> MDLTVEPNLHSLITSTTHKWIFVGGKGGVGKTTSSCSIAIQMALSQPNKQFLLISTDPAHNLSDAFGEKFGKDARKVTGMNNLSCMEIDPSAALKDMNDMAVSRANNNGSDGQGDDLGSLLQGGALADLTGSIPGIDEALSFMEVMKHIKRQEQDEGETFDTVIFDTAPTGHTLRFLQLPNTLSKLLEKFGEITNKLGPMLNSFMGAGNVDISGKLNELKANVETIRQQFTDPDLTTFVCVCISEFLSLYETERLIQELISYDMDVNSIIVNQLLFAENDQEHNCKRCQARWKMQKKYLDQIDELYEDFHVVKMPL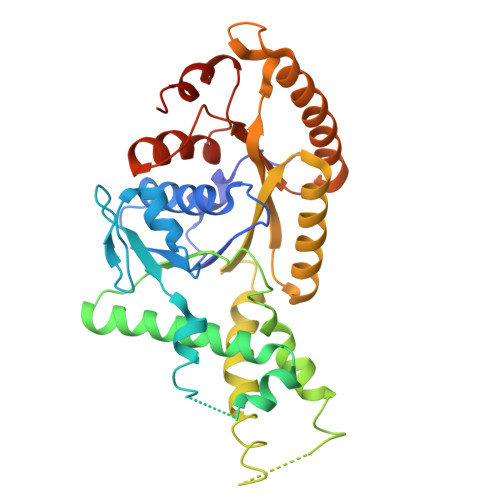CAGEIRGLNNLTKFSQFLNKEYNPITDGKVIYELEDKELEHHHHHH> GMTNVGRPIETHAITVGQGSDARSIAALVRAPAQDERPTCIWLGGYRSDMTGTKALEMDDLAASLGVGAIRFDYSGHGASGGAFRDGTISRWLEEALAVLDHFKPEKAILVGSSMGGWIALRLIQELKARHDNPTQVSGMVLIAPAPDFTSDLIEPLLGDRERAELAENGYFEEVSEYSPEPNIFTRALMEDGRANRVMAGMIDTGCPVHILQGMADPDVPYQHALKLVEHLPADDVVLTLVRDGDHRLSRP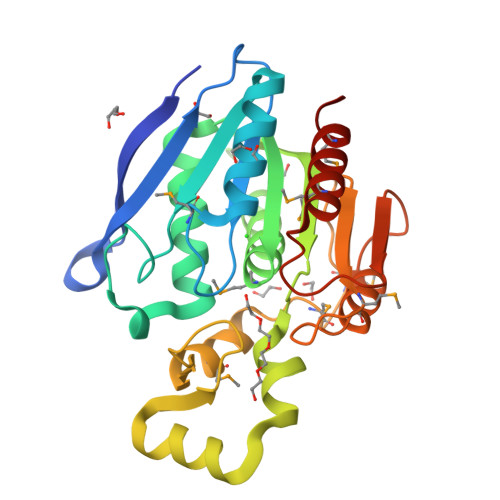QDIDRMRNAIRAMIEPRP> IVGGQDATRGMFPYQLSLQHMGAGWYHTCGAILLAANKALTAAHCTEGREGFRVLAGAHVLPANDQEQESDVASVTEHPEFDRFGPGIPNDVATMALATAINAAGNVGYATLAAANAPD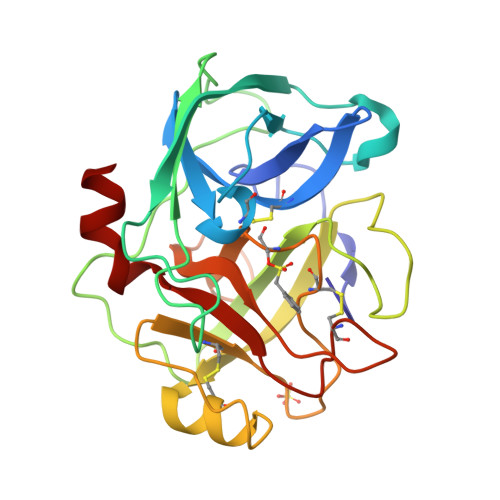YAGDQARLSGWGKLHGADDGIADTLQYVVTTVRSTADCNARMPEHIQNVMDQHICVHSDTGTTGSCQGDSGGPMTHGASGSGNVIGVTSWGIGNPVESCLPDFPSVYARVSYFRAWIDAN N-(4-{[4-(pyrrolidin-1-yl)piperidin-1-yl]sulfonyl}benzyl)-2H-pyrido[4,3-e][1,2,4]thiadiazin-3-amine 1,1-dioxide | C22 H28 N6 O4 S2 | 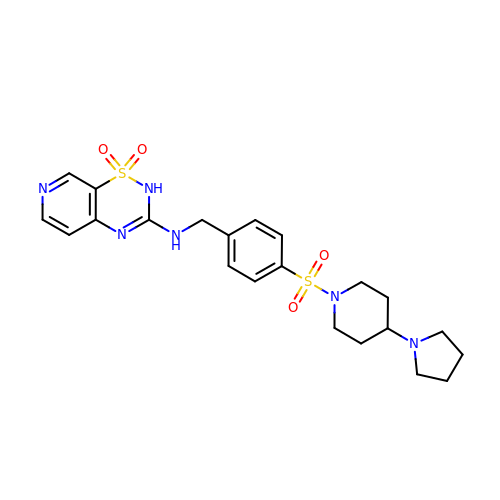BCPZRYGPLBZKEZ-UHFFFAOYSA-N pentan-3-yl 2-acetamido-2,4-dideoxy-alpha-L-threo-hex-4-enopyranosiduronic 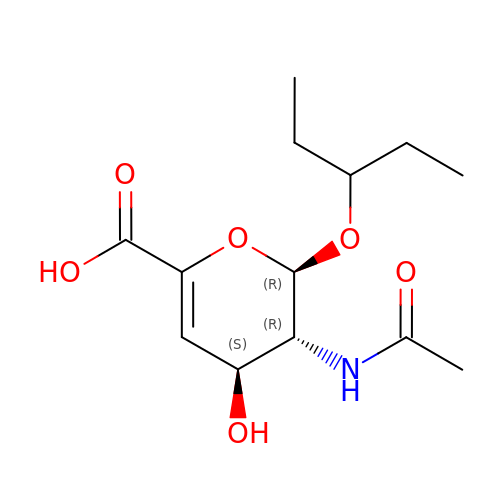acid | C13 H21 N O6 | UUULUCUBSUJBNQ-UFGOTCBOSA-N However, intestinal bacterial GUSs cleave the attached glucuronic acid for use as a carbon source, allowing potentially toxic compounds to re-enter the enterohepatic circulation. However, microflora-encoding β-glucuronidases (GUSs) are notorious for reversing the glucuronidation to release SN-38 in the intestinal lumen and thus represent the major cause of undesirable effects. GUS contains a deep enzyme active site (the two catalytic glutamates lie ~12 Å below the protein surface). To understand the underlying structural basis, we prepared C6-propyl, -hexyl, and -nonyl UIFGs (2–4, respectively) and resolved the eight X-ray crystal structures of 1–4 bound to EcGUS or Bifidobacterium dentium GUS (BdGUS).

Particularly, C6-nonyl UIFG had 23,300-fold higher potency for EcGUS than for HsGUS (Ki = 4.5 nM for EcGUS vs. 105 μM for HsGUS). The IC50 was as follows: 2, 1.2 μM; 3, 18.6 nM; and 4, 3.69 nM. Consistent with the aforementioned Ki values, 4 was the most potent inhibitor. Furthermore, EcGUS contains a narrower aglycone-binding site than LgGUS and BdGUS. Taking the comparison between EcGUS and HsGUS as an example, the aglycone-binding site of EcGUS is surrounded by five hydrophobic residues, namely Phe365, Leu361, Val446, Met447, and Phe448, which are located in loops 3 and 5, whereas the site of HsGUS is surrounded by Ser485loop 5, Tyr505loop 6, His509loop 6, and Thr599loop 8. This difference explains why substitution with an alkyl group at C6 of UIFG remarkably enhanced its binding affinity and selectivity for EcGUS. The alkyl substituent of the inhibitors therefore facilitated an increase in hydrophobic contacts with nonpolar residues of loops 3 and 5 in EcGUS, e.g., such as Leu361, Phe365 in loop 3, and Val446, Met447, and Phe448 in loop 5. Interestingly, owing to the longer alkyl chains of 3 and 4, Phe448 rotated outward in EcGUS/3 and EcGUS/4 and thus increased the hydrophobic contact area. This additional hydrophobic interaction might have compensated for the binding energy loss owing to the absence of the water-mediated H-bond network, leading to the observed lower Ki values of 2–4 for EcGUS compared with other GUSs. Similar to the previous trend, the entropy contribution of 3 and 4 increased with the length of alkyl chain (–TΔΔS2–3 = –1.32 kcal mol−1 and –TΔΔS2–4 = −1.34 kcal mol−1 for EcGUS), while the enthalpy contribution decreased (ΔΔH2–3 = +0.04 kcal mol−1 and ΔΔH2–4 = +0.99 kcal mol−1 for EcGUS).

> SHMLRPVETPTREIKKLDGLWAFSLDRENCGIDQRWWESALQESRAIAVPGSFNDQFADADIRNYAGNVWYQREVFIPKGWAGQRIVLRFDAVTHYGKVWVNNQEVMEHQGGYTPFEADVTPYVIAGKSVRITVCVNNELNWQTIPPGMVITDENGKKKQSYFHDFFNYAGIHRSVMLYTTPNTWVDDITVVTHVAQDCNHASVDWQVVANGDVSVELRDADQQVVATGQGTSGTLQVVNPHLWQPGEGYLYELCVTAKSQTECDIYPLRVGIRSVAVKGEQFLINHKPFYFTGFGRHEDADLRGKGFDNVLMVHDHALMDWIGANSYRTSHYPYAEEMLDWADEHGIVVIDETAAVGFNLSLGIGFEAGNKPKELYSEEAVNGETQQAHLQAIKELIARDKNHPSVVMWSIANEPDTRPQGAREYFAPLAEATRKLDPTRPITCVNVMFCDAHTDTISDLFDVLCLNRYYGWYVQSGDLETAEKVLEKELLAWQEKLHQPIIITEYGVDTLAGLHSMYTDMWSEEYQCAWLDMYHRVFDRVSAVVGEQVWNFADFATSQGILRVGGNKKGIFTRDRKPKSAAFLLQKRWTGMNFGEKPQQGGKQ;> RPVETPTREIKKLDGLWAFSLDRENCGIDQRWWESALQESRAIAVPGSFNDQFADADIRNYAGNVWYQREVFIPKGWAGQRIVLRFDAVTHYGKVWVNNQEVMEHQGGYTPFEADVTPYVIAGKSVRITVCVNNELNWQTIPPGMVITDENGKKKQSYFHDFFNYAGIHRSVMLYTTPNTWVDDITVVTHVAQDCNHASVDWQVVANGDVSVELRDADQQVVATGQGTSGTLQVVNPHLWQPGEGYLYELCVTAKSQTECDIYPLRVGIRSVAVKGEQFLINHKPFYFTGFGRHEDADLRGKGFDNVLMVHDHALMDWIGANSYRTSHYPYAEEMLDWADEHGIVVIDETAAVGFNLSLGIGFEAGNKPKELYSEEAVNGETQQAHLQAIKELIARDKNHPSVVMWSIANEPDTRPQGAREYFAPLAEATRKLDPTRPITCVNVMFCDAHTDTISDLFDVLCLNRYYGWYVQSGDLETAEKVLEKELLAWQEKLHQPIIITEYGVDTLAGLHSMYTDMWSEEYQCAWLDMYHRVFDRVSAVVGEQVWNFADFATSQGILRVGGNKKGIFTRDRKPKSAAFLLQKRWTGMNFGEKPQQGGKQ>[4x]MASLNCHDKCSTTTQSDINLKDELLSSTSIECRPGNDLLESLHKEQNRWYSETKTFSDSSQHTGRGFEKYWFCYGIKCYYFVMDR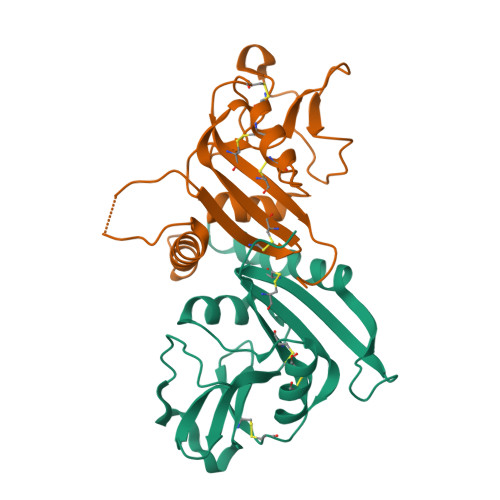KTWSGCKQTCQISSLSLLKIDNEDELKFLKLLVPSDSYWIGLSYDNKKKDWAWINNGPSKLALNTMKYNIRDGGCMLLSKTRLDNDNCDKSFICICGKRLDKFPH benzo[g][1]benzothiole-2-carboxylic acid | C13 H8 O2 S | 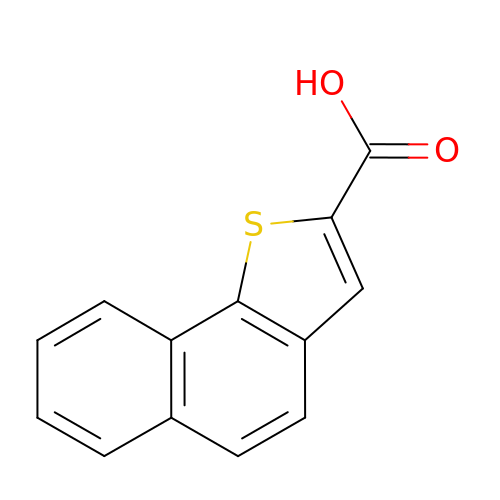KRSFUJUZIQCOHU-UHFFFAOYSA-N>GPMEEPSLLDAHNVRVVGMGSELVVLGHGFGTDQSVWKHVIPHLVDDYRVILFDNMGAGTTDPEFFSFSRYSTLHGYADDLLSILEELEVESCIYVGHSVAGMVGCLASLERPEIFT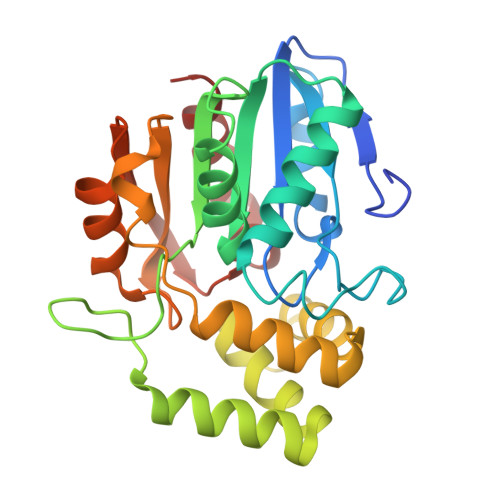KIITLSASPRYLNDRDYFGGFEQDDLNQLFEAMQSNFKAWVSGFAPLAVGSDIDSMAVQEFGRTLFNIRPDIAFSVAKTIFQSDLRIMLPKVTVPCHILQSSKDLAVPLVVADYLHHALGGPTIVEVLPTEGHLPQLSSPDIIIPVLKRHLAGSL[2x]>[4x]IKDNSILDMRYENNKFIDISGYGSNISINGDVYIYSTNRNQFGIYSSKPSEVNIAQNNDIIYNGRYQNFSISFWVRIPKYFNKVNLNNEYTIIDCIRNNNSGWKISLNYNKIIWTLQDTAGNNQKLVFNYTQMISISDYINKWIFVTITNNRLGNSRIYINGNLIDEKSISNLGDIHVSDNILFKIVGCNDTRYVGIRYFKVFDTELGKT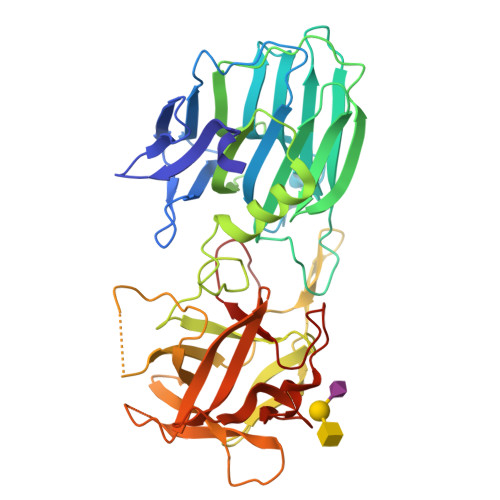EIETLYSDEPDPSILKDFWGNYLLYNKRYYLLNLLRTDKSITQNSNFLNINQQRGVYQKPNIFSNTRLYTGVEVIIRKNGSTDISNTDNFVRKNDLAYINVVDRDVEYRLYADISIAKPEKIIKLIRTSNSNNSLGQIIVMDSIGNNCTMNFQNNNGGNIGLLGFHSNNLVASSWYYNNIRKNTSSNGCFWSFISKEHGWQEN>[2x]MFIINSDFHRGNMEQYQKAQKLSFDPAELLRTSLNVGDIVLLKQCTSELTMCVNLPQSTTDPRYTFAKKDGTLVYAMKNSVILRIPKDLPEEVNQLLKRESNHPYQKIGTIKNSSNETEILPVLTRQLIVSFTLATFTKFAWTQLPIVLKKLELIHRYLQDSRGSKHVNFMSLVRIIKNLNIKEATDAINGDAYVRKVIDESMSVVNKSIDPTTLLATYWGVREQQQNNLWGSVYTNTALLSPTTVAVLPLKKAHLFYQEVITRLESNDYQEIKAFAKLVNDKDYHSIAKRYDYIRTLLNDYAAGNIEENAVLTTIISKIFRHIDMYRDQDVTRSLCGKLLVEISPQSNSSNFILGNWDLNIPKSSGISSVEQKLYDTAMPTIVSDTDRYDFGDMPVFCIDSEDAHEINDGISIEELDGVRSRIHIHIADPAGLFPESFDYTKSGISDDVLRVSLKRAFTTYLPDLVVPMLPKSFCNRADLGKHDRKTETISFSFELVNKEDGGLHVDYDTFQVRLGIVSNFPKVTYDKVDSILNGDDNSLPSKQKKQLELLHTLATKLLHKRIHDDNAVVFGDGFNKGLVSLSPDDDGELCIPTFYDQSQTKSTLLVSEFMILTNKLCAAFFQENKIPGVYRCYNGLNLGNQAKAQFELLKENIKLGKLPSLKDITKISSQLSSSFYSPFPLPHKMIGNTAYLTVTSPMRRGPDLINHLQLHRFLKKLPLCFKQEYLDQYVWSFQARADILKIFQRHSSTYWTLKHLEQSGTKTHDVIVTSVPQNGTVNCLFPEYSYARGTLKLDPAMKKIPRIGDTIRHCKVESIHPLDGILTLTHVNRK

The mtEXO complex is composed of two subunits: the nucleotide triphosphate (NTP)-dependent RNA helicase Suv3 and the 3′-to-5′ exoribonuclease Dss13. Dss1 individually has low RNase activity, and the robust nucleolytic activity of the entire degradosome complex nearly completely depends on ATP, an unprecedented feature that is not found in other known RNA-degrading systems. To understand the structure and mechanism of the yeast mitochondrial RNA degradosome, we present crystal structures of Dss1 nuclease and the mtEXO complex of the yeast Candida glabrata (Cg). Our structural analysis revealed the architecture of the Cg-mtEXO complex, in which the helicase motor feeds the 3′ end of the RNA into the catalytic channel of Dss1 for efficient and processive degradation.

We then designed several deletion constructs and obtained stable preparations of the Cg-Dss1 protein with a deletion of 69 N-terminal residues (Cg-Dss170–900). We also introduced an inactivating point substitution (D477N) in the active site of the RNB domain to prevent RNA degradation during crystallization. We obtained crystals of this variant of Cg-Dss1 (Cg-Dss170–900 D477N) that belonged to space group P 1 and diffracted X-rays to 2.7 Å resolution at a synchrotron source. The structure was solved using crystals of selenomethionine-substituted protein and single-wavelength anomalous diffraction (SAD). Two copies of the protein molecule were present in the asymmetric unit. In summary, the structure of Dss1 shows that it is a special member of the RNase II family in which N-terminal domains - β-barrel, WH and HTH replace the typically observed CSD1 and CSD2. At the N-terminus a β-barrel domain is present (residues 92–170 of Cg-Dss1) with a patch of positively charged residues facing the RNA-binding channel. DALI16 search revealed that it is a winged helix (WH) domain. The second domain that is unique to Dss1 is a double HTH domain (residues 320–419 in Cg-Dss1). The catalytic domain of Cg-Dss1 is very similar to the RNB domains of the other RNase II family members and can be superimposed on them with an RMSD between 1.6 and 2.0 Å.4-octylphenyl 6-O-sulfo-alpha-D-glucopyranoside | C20 H32 O9 S | 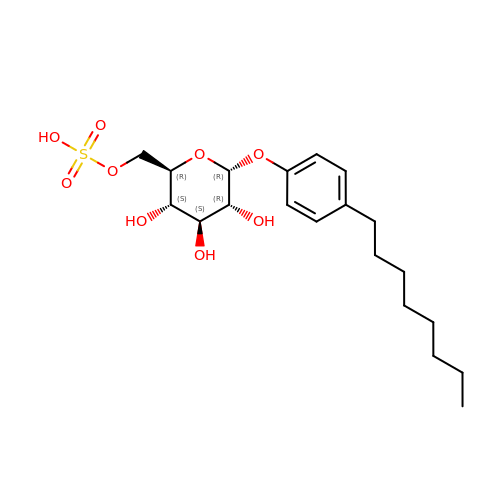YVWGSDRSYRDYCF-OBKDMQGPSA-N5-[(3S)-1,2-dithiolan-3-yl]pentanoic acid | C8 H14 O2 S2 | 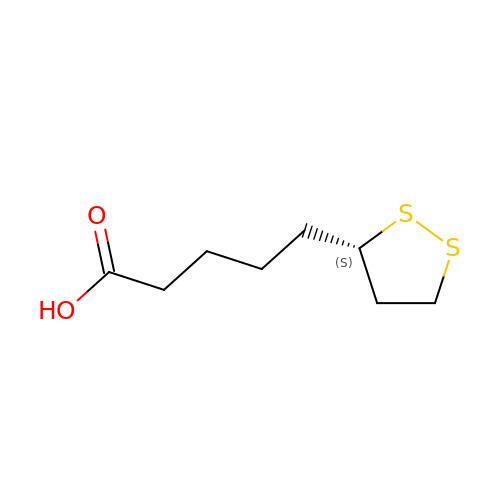AGBQKNBQESQNJD-ZETCQYMHSA-N1-(4-((1H-pyrrolo[2,3-b]pyridin-4-yl)oxy)phenyl)-3-(5-(4-methylpiperazin-1-yl)naphthalen-2-yl)urea | C29 H28 N6 O2 | 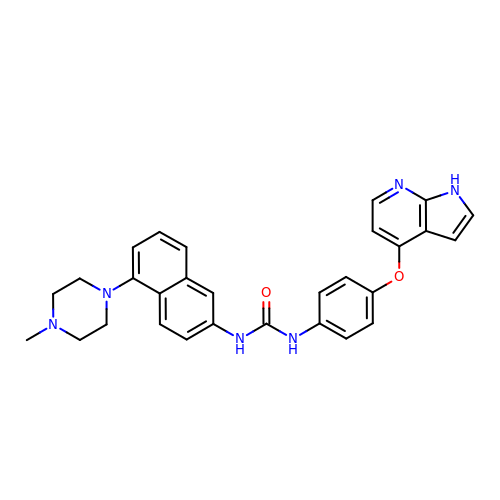WQRGBJPKMNUGRL-UHFFFAOYSA-N AJLec was purified from A. japonica and identified as a Ca2+-dependent and galactose-specific lectin (18.5 kDa) forming a disulfide-bonded dimer. Hemagglutination inhibition assay, ITC analysis, and glycoconjugate microarray revealed its strict specificity for β-linked terminal galactose, but not for GalNAc. The primary structure of AJLec was not homologous with that of any known lectins. Accordingly, AJLec was assumed to be a novel type of lectin with a unique structure and specificity.

The crystal structure of AJLec in complex with lactose was determined in the orthorhombic space group P212121 with unit cell parameters a = 38.1 Å, b = 79.7 Å, and c = 106.0 Å. Two polypeptide chains were found to be present in the asymmetric unit, and a total of 164 amino acid residues per polypeptide chain were observed. There are two disulfide bonds at Cys3 and Cys122 between the two chains in the asymmetric unit. Therefore, the dimer structure, formed due to the formation of the disulfide bonds, was supposed to be a functional dimer in solution. The dimer structure forms a helical-bar like shape, where lactose binding sites are located on both of its termini. The protomer structure of AJLec was composed of a core structure with seven β-sheets and three surrounding helices and loops. The seven β-sheets formed small jelly-roll type β-sandwich folds. A lactose molecule in the site was bound to a Ca2+ ion, where its glucose residue was quite solvent exposed whilst its galactose residue was mainly buried in the binding site groove. β-galactose residue in lactose is held by two coordinate bonds with Ca2+ ion and two hydrogen bonds with side chain nitrogen atoms of Arg64; hydroxyl groups at positions 2, 3, and 4, and oxygen at position 5 in the β-galactose residue form hydrogen and coordinating bonds in the site. The binding of β-galactose residues was further stabilized by hydrophobic interactions between the hydrophobic face of the β-galactose residue in the lactose and side chains of Phe67, Tyr97, and Phe103. In addition, the Ca2+ ion coordinately bound sidechain oxygen atoms of Glu141, Asp150, and Asn151, and main chain oxygen atoms of Met147 and Cys48, present in these sites.

>[2x]QRCGGWVKLNTAPVCFSAKGNRPGSFTPSHHGFLKSVKLRHLRGLVTCQSSTDAHDSYWGCKNRNGFHNYPLNVFVTDKHNKVMFPKTGATYYLDPYVIKNRFYGVQGYNAMSPELVLQHGCNSPSDYIGPDSQLRVWYGEDLYNTMESDNSGKVCADVFGYFV> MLNSNIYIIIYGGIIMYSIMIIIQMFLYNFSNKIYIEVEINKYILSKNNIDIYWIICNCTIIIIITTLNHIINKIGIYNMIEYNICYWLIGTGLGLYISPFIVFGYKFFVYIMDLNNYSLNIYHNNNKMNDIQQIYNGTNYNDTMIFFIKDINNIFTIYRSINFFMNWLYQMIYYGVRMWLVFVLHSFSLGSFGELITVITDNNLIFNVFYIGLLGLGFILYLIV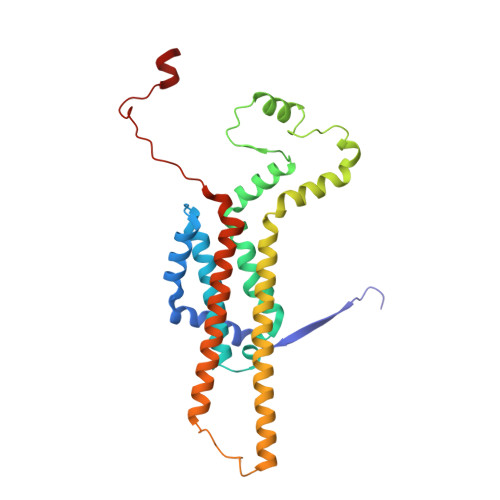IFYLGIQIYVYISFSLSFLHSTILLFLVNYIPHYNNKSIFNTFTNKSIY>GAMGSSPNYDKW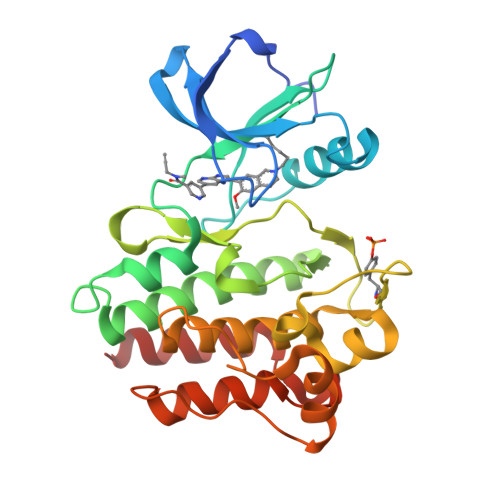EMERTDITMKHKLGGGQYGEVYEGVWKKYSLTVAVKTLKEDTMEVEEFLKEAAVMKEIKHPNLVQLLGVCTREPPFYIITEFMTYGNLLDYLRECNRQEVNAVVLLYMATQISSAMEYLEKKNFIHRDLAARNCLVGENHLVKVADFGLSRLMTGDTYTAHAGAKFPIKWTAPESLAYNKFSIKSDVWAFGVLLWEIATYGMSPYPGIDLSQVYELLEKDYRMERPEGCPEKVYELMRACWQWNPSDRPSFAEIHQAFETMFQES[2x]> 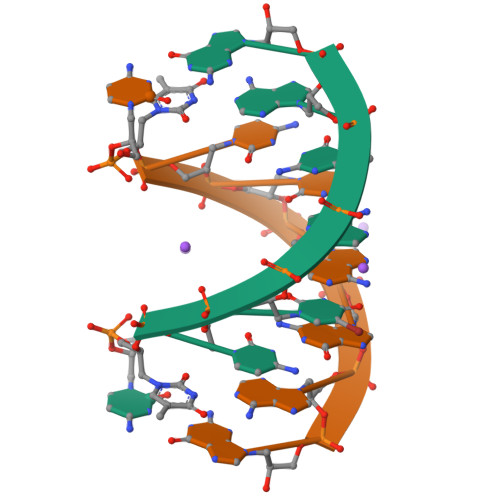CXCUAGAG Holliday junction resolution is a crucial process in homologous recombination and DNA double-strand break repair. Holliday junction (HJ) is a four-way structured DNA intermediate formed during the homologous recombination. Canonical HJ resolvases introduce two symmetrical nicks across the junction center by functioning as homodimers, and exhibit strong structure- and sequence-specificities in HJ cleavage. The RNase H-like enzymes, including RuvC and MOC1, typically feature three or more conserved carboxylates, known as the DDE motif, in their active sites.

First, to prevent spontaneous cleavage, the crystals of MOC1/nHJ complex were initially grown in the presence of Ca2+ ions, which were subsequently depleted by soaking in an EGTA containing solution. The structure of MOC1/nHJ complex in its ground state was determined at a resolution of 2.0 Å. The inspection of electron density map confirmed the depletion of Ca2+ ions, which were replaced by water molecules within both active sites. The overall configuration of catalytic site closely resembles that of our previous reported free MOC116, but differs significantly from the Ca2+ bound state, particularly in residues D115, D117, E174 and E257. These observations thus suggest that the active site configuration has been reset to its initial ground state following the depletion of Ca2+ ions.

>GWVIGVDPDIGGAIAVLSPDGSSQVFDNPFVHIVVSEVIRKRLDTKSIIQLLRGLDAPPGTTAYIEKSSPFPTDGKQGWWSTGFSYGLWIASLVASGFSVVPIASQTWKAYFGLMRSETPKDDSRQAASILFPDKDQSLKLKKHHGRAEALLLAAYGKGLVLP[2x]>[2x]MKFILAEKFTFDPLSNTLIDKEDSEEIIRLGSNESRILWLLAQRPNEVISRNDLH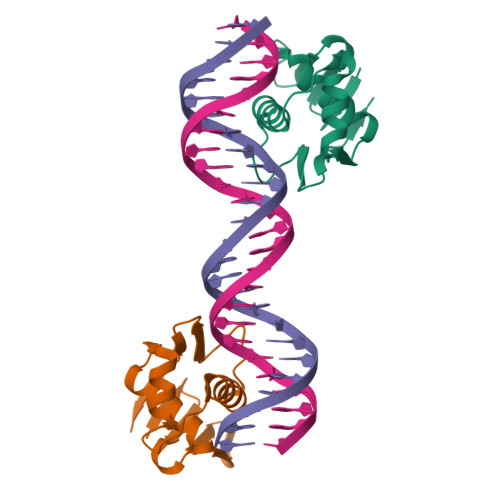DFVWREQGFEVDDSSLTQAISTLRKMLKDSTKSPQYVKTVPKRGYQLIARVETV>[2x]GMKNAPLTLNFGSVRLPVSADGLLHAPTAQQQLGLTQSWEAALVEHGLPETYRDFGAGPEAAVSVPDFVAL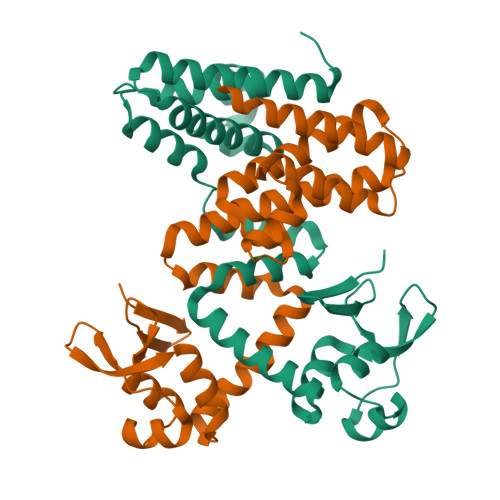AFALDTPEARRWQKRARELLARAMQGDVRVAAQIAERNPEPDARRWLAARLESTGARRELLATVARHGGEGRVYGQLGSISNRTVLGKDSASVRQERGVKATRDGLTSAELLRLAYIDTVTARAIQESEARGNAAILTLHEQVARSERQSWERAGQVQRVG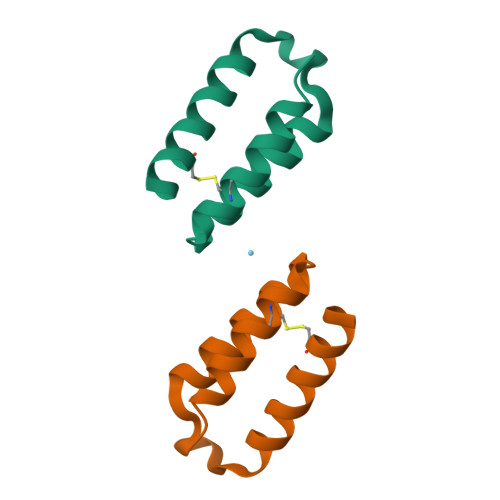> DDKAACADGIAAVKARVEKLAPEAVPQKLKRALKIAEREQGEGEFDECLEALDDAKRALPK>MSAKSRTIGIIGAPFSKGQPRGGVEEGPTVLRKAGLLEKLKEQECDVKDYGDLPFADIPNDSPFQIVKNPRSVGKASEQLAGKVAEVKKNGRISLVLGGDHSLAIGSISGHARVHPDLGVIWVDAHTDINTPLTTTSGNLHGQPVSFLLKELKGKIPDVPGFSWVTP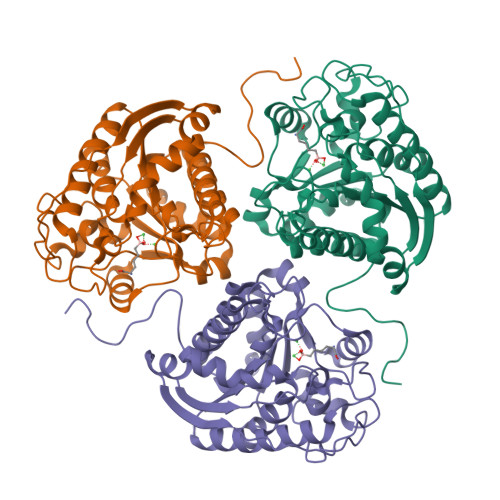CISAKDIVYIGLRDVDPGEHYILKTLGIKYFSMTEVDRLGIGKVMEETLSYLLGRKKRPIHLSFDVDGLDPSFTPATGTPVVGGLTYREGLYITEEIYKTGLLSGLDIMEVNPSLGKTPEEVTRTVNTAVAITLACFGLAREGNHKPIDYLNPPK[2x]> LSTEIRKAIEDAIESAPVV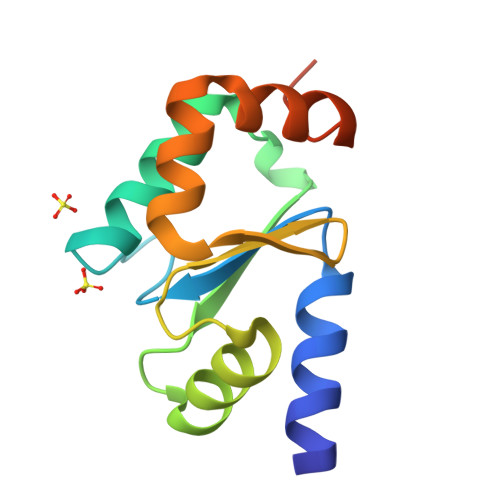LFMKGTPEFPKCGFSRATIGLLGNQGVDPAKFAAYNVLEDPELREGIKEFSEWPTIPQLYVNKEFIGGCDVITSMARSGELADLLEEAQALVPEEEEETKDR> SCC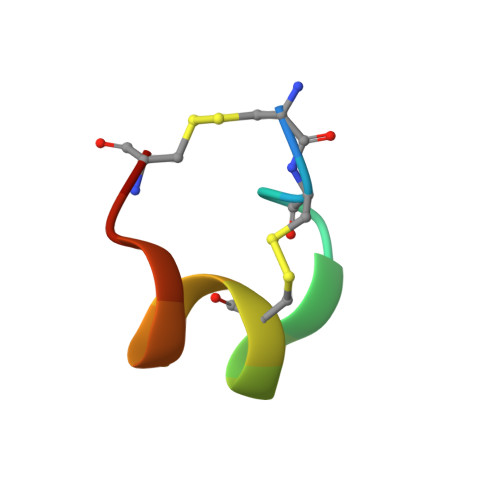ARNPACRHNHPCV>[8x]MAVPEVVVEGVVFPPVARPPGSAGSHFLGGAGVRGIEIGGNFIKFTAIGVYLEDAAVSALAKKWAGKTADELASDAAFFRDVVTGDFEKFTRVTMLLPLTGEQYAGKVTENCVAFWKAVGLYTDAEGVAVEKFKEAFKPETFPPGASILFTHSSTGVLTVAFSKDSSVPASGGVAIENKHLCEAVLESIIGEHGVSPAAKLSLAARVSELLTKGTAGAADAPQAEPVSVTA

Chalcone synthase (CHS) and chalcone isomerase (CHI) catalyze the first two committed steps of the flavonoid pathway that plays a pivotal role in the growth and reproduction of land plants, including UV protection, pigmentation, symbiotic nitrogen fixation, and pathogen resistance. Based on the obtained X-ray crystal structures of CHS, CHI, and chalcone isomerase-like protein (CHIL) from the same monocotyledon, Panicum virgatum, along with the results of the steady-state kinetics, spectroscopic/thermodynamic analyses, intermolecular interactions, and their effect on each catalytic step are proposed. The production of these value-added products also offers the prospect of increasing the value of the crop, especially because many of these compounds are soluble and readily extracted. This study characterized the enzymes involved in the first two committed steps of the flavonoid pathway, CHS and CHI, and the non-catalytic protein CHIL. Through crystal structure, molecular docking, mutagenesis, kinetic analyses, ITC, and FRET analysis, our study provides evidence supporting a revised catalytic reaction mechanism for monocot CHS and CHI and identified an intermolecular interaction of CHS with both CHI and CHIL in a non-competitive manner.

Our attempt to produce a binary complex with the substrate was only successful for SbCHI. From the early stage of refinement, the electron density corresponding to liquiritigenin that had been added to the crystallization buffer was clearly identified. The bound liquiritigenin, the product of isoliquiritigenin, a type II substrate, was surrounded by 34RGI36 from β3a, 44FTAI47 from β3a, 104YAGKVTEN111 from α4, and 147SI148 from α6. Notably, the molecule was surrounded with predominantly hydrophobic residues: Ile-38, Ile-36, Phe-45, and Leu-99. In addition, a hydrogen bond was established between the sidechain of Lys-107 and the C2′ hydroxyl group of the bound liquiritigenin. The overall structure of SbCHI was very similar to that of PvCHI, with an RMSD of 0.66 Å. The noticeable differences between SbCHI and PvCHI were observed in the loops between β3a and β3b and β2 and β3a. In addition, α8 of PvCHI was shorter, as the C-terminus of PvCHI was more disordered than that of SbCHI. The Vmax of SbCHI was 2889 μM s−1 and 0.238 μM s−1 for naringenin chalcone and isoliquiritigenin, respectively. The Km was 16.55 μM and 1.585 μM for naringenin chalcone and isoliquiritigenin, respectively.>MLLEAPVYKEIFGAVTIHEVQKVIKMDTETEEVPIYTISNIPREKIYDLLGKMAVIVPMKNEKLHLVDGVLKAIPHKCPIIIVSNSKREGPNRYKLEVDLIRHFYNLTHSKIIMIHQKDPGLAKAFKEVGYTDILDENGMIRSGKGEGMLVGLLLAKAIGAEYVGFVDADNYIPGAVNEYVKDYAAGFLMSESEYTMVRLHWRHKPKVTKGTLYFKKWGRVSEITNHYLNLLVSEHTAFETTIMVTGNAGEHAMTMKLAEILPFSTGYSIEPYEIVYILERFGKWENVEEFKDVFDQGIEIFQIETLNPHFHEDKGKEHVKEMLLLSLATIYHSKLATDNLRKRILKDLRDHGILGENEEPPKPL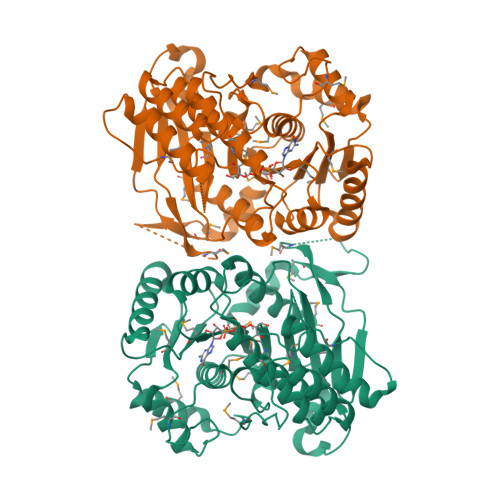VMRPIKEIPIKEWMDIVEGNSETLLRFEL[2x]> GSHMNVFNPAQFRAQFPALQDAGVYLDSAATALKPEAVVEATQQFYSL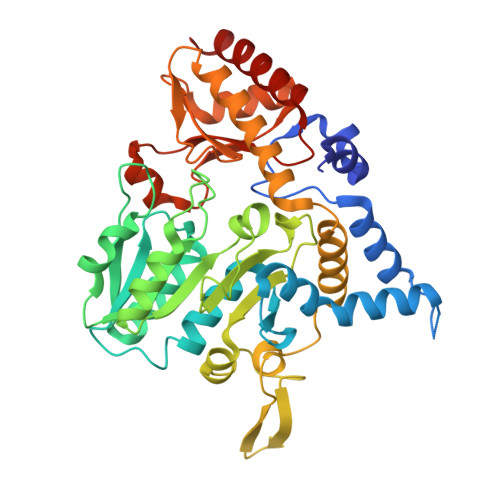SAGNVHRSQFAEAQRLTARYEAAREKVAQLLNAPDDKTIVWTRGTTESINMVAQCYARPRLQPGDEIIVSVAEHHANLVPWLMVAQQTGAKVVKLPLNAQRLPDVDLLPELITPRSRILALGQMSNVTGGCPDLARAITFAHSAGMVVMVDGAQGAVHFPADVQQLDIDFYAFSGHKLYGPTGIGVLYGKSELLEAMSPWLGGGKMVHEVSFDGFTTQSAPWKLEAGTPNVAGVIGLSAALEWLADYDINQAESWSRSLATLAEDALAKRPGFRSFRCQDSSLLAFDFAGVHHSDMVTLLAEYGIALRAGQHCAQPLLAELGVTGTLRASFAPYNTKSDVDALVNAVDRALELLVD>MTSAEMTSPNNNSEHQAIAKMRTMIEGFDDISHGGLPIGRSTLVSGTSGTGKTLFSIQFLYNGIIEFDEPGVFVTFEETPQDIIKNARSFGWDLAKLVDEGKLFILDASPDPEGQEVVGGFDLSALIERINYAIQKYRARRVSIDSVTSVFQQYDASSVVRRELFRLVARLKQIGATTVMTTERIEEYGPIARYGVEEFVSDNVVILRNVLEGERRRRTLEILKLRGTSHMKGEYPFTITDHGINIFPLGAMRLTQRSSNVRVSSGVVRLDEMCGGGFFKDSIILATGATGTGKTLLVSRFVENACANKERAILFAYEESRAQLLRNAYSWGMDFEEMERQNLLKIVCAYPESAGLEDHLQIIKSEINDFKPARIAIDSLSALARGVSNNAFRQFVIGVTGYAKQEEITGLFTNTSDQFMGAHSITDSHISAITDTIILLQYVEIRGEMSRAINVFKMRGSWHDKAIREFMISDKGPDIKDSFRNFERIISGSPTRITVDEKSELSRIVRGVQEKGPES[6x]

The circadian clock of the cyanobacterium Synechococcus elongatus can be reconstituted in vitro by three proteins, KaiA, KaiB and KaiC. Homo-hexameric KaiC displays kinase, phosphatase and ATPase activities; KaiA enhances KaiC phosphorylation and KaiB antagonizes KaiA. The crystal structure of KaiC from S. elongatus revealed a hexamer in the shape of a double doughnut with approximate dimensions 100×100 Å, whereby the N-terminal CI and C-terminal CII halves of subunits are joined by a 15-amino acid linker. Two phosphorylation sites (P-sites), T432 and S431 that are both located in the CII half were identified in KaiC.

To analyze the phosphorylation patterns of KaiC P-site mutants and to visualize potential conformational variations in the vicinity of bound ATP and residues 432 and 431 at hexamer subunit interfaces, we determined crystal structures of the S. elongatus KaiC single mutants T432A (TSa), S431A (TaT), S431D (TdT), and T426N (nST) and the double mutants T426A/T432A (aSa) and S431A/T432E (Tae). b KaiC mutations xyz or mutants KaiCxyz are sequentially shown in order of sites x = 426, y = 431, and z = 432 where the wild-type residue is in upper case and mutated residues are shown in lower case, i.e. Tsa or KaiCTSa, where the residue at position 426 is T, the residue at position 431 is S, and the residue at position 432 is mutated to A. Interestingly, in the structure of KaiCTSa, A432 has moved closer to the γ-phosphate group of ATP: average distance 5.6 Å vs. 8.2 Å (wt-KaiC). One may have expected the above KaiCTSa mutant to represent the state before dephosphorylation of the second P-site (pS431). Instead its structure is more representative of the initial phosphorylation event. The combined structural data expose subtle changes in the orientations of the H423-I433 loop region harboring phosphorylated residues relative to the γ-phosphate of ATP compared with the structure of wt-KaiC.>CGVFGIWGHEEAPQITYYGLHSLQHRGQEGAGIVATDGEKLTAHKGQGLITEVFQNGELSKVKGKGAIGHVRYATAGGGGYENVQPLLFRSQNNGSLALAHNGNLVNATQLKQQLENQGSIFQTSSDTEVLAHLIKRSGHFTLKDQIKNSLSMLKGAYAFLIMTETEMIVALDPNGLRPLSIGMMGDAYVVASETCAFDVVGATYLREVEPGEMLIINDEGMKSERFSMNINRSICSMEYIYFSRPDSNIDGINVHSARKNLGKMLAQESAVEADVVTGVPDSSISAAIGYAEATGIPYELGL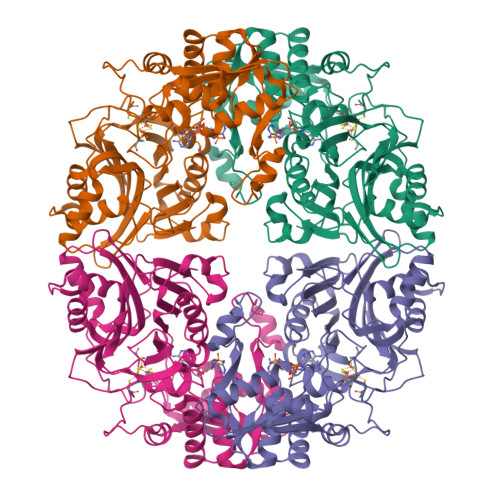IKNRYVGRTFIQPSQALREQGVRMKLSAVRGVVEGKRVVMVDDSIVRGTTSRRIVTMLREAGATEVHVKISSPPIAHPCFYGIDTSTHEELIASSHSVDEIRQEIGADTLSFLSVEGLLKGIGRKYDDSNCGQCLACFTGKYPTEIYQDTVLPHVKEAVLTK[4x]> GDQVEQSPSALSLHEGTDSALRCNF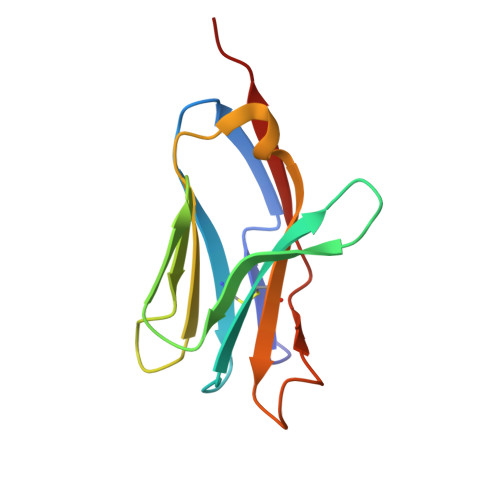TTTMRSVQWFRQNSRGSLISLFYLASGTKENGRLKSAFDSERARYSTLHIRDAQLEDSGTYFCAAEASSGSWQLIFGSGTQLTVMPVT> MNNSSELIAVINGFRNSGRFCDISIVINDERINAHKLILSGASEYFSILFSNNFIDSNEYEVNLSHLDYQSVNDLIDYIYGIPLSLTNDNVKYILST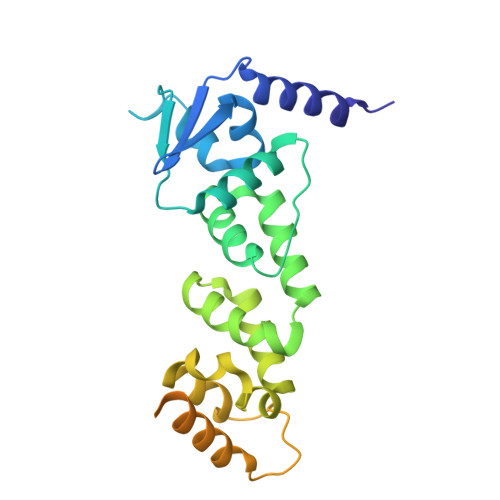ADFLQIGSAITECENYILKNLCSKNCIDFYIYADKYNNKKIESASFNTILQNILRLINDENFKYLTEESMIKILSDDMLNIKNEDFAPLILIKWLESTQQSCTVELLRCLRISLLSPQVIKSLYSHQLVSSIYECITFLNNIAFLDESFPRYHGSKHHHHHH>MAFNPAPKAVQENHHVDYVIRFNYGDIDTPEAIKKFEVLLLELSEVGLQTEVRQGDENSLFVFVRAASKKKLKRAVYQSRVRDWLYGVRNTEPEPASSAKPQSEAERLLVIYHLITVPKAEGGAGITPRHGEWKNVDAIFPLHDEETNRQCMREWSKKTFLSTEDLDRIRNTFGEHVGFYFAFLQSYFRFLMFPAAFGFSCWLLLGSFSIIYTVVNCLWCIVFIEYWKRQEEDLSCRWQTKGVSAVHEKRAEFKPEKEIRDESTGEVRGVFPATKRMYRQLLQVPFALLAAVALGAIIATCFAIEIFISEVYNGPLKGYLVFIPTILVSALIPTMSAVLLTVATKLNDYENYETQDAYKVALTQKIFVVNFITSYLPIILTAFVYVPFASRIVPYLDVFHLTVRPFVSKEHAIKARTEFSINPDRLRKQVIYFTVTAQIVGFALETIVPFVKQRVFREYKEYTKKQHAKAEPGNGAGEKKTVSLGDDEDEARFLTRVRNEAELEDYDVTDDLREMCIQFGYLALFSPVWPLVPVSFLINNWVELRSDFFKICVECKRPWPQRADTIGPWLDSLGFLSWVGSITSSALV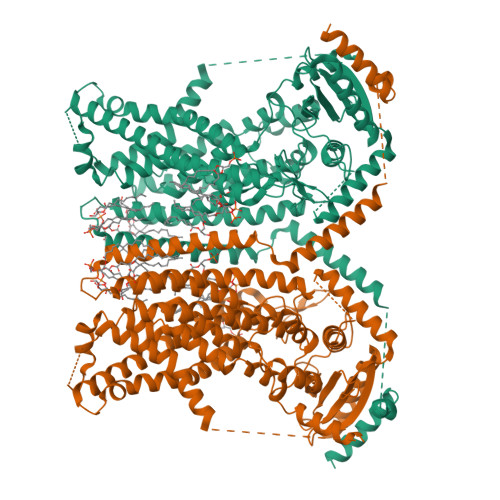YMFSNGHEGPNGEPTTIRCWALLLTIFFSEHLYLIVRYAVRSALAKLEPPNTRRERIERFMMRKRYLDTVLSAESDDDADEVKGVVSSIPPSEITRESLEQDARDWSKQGTDPTERFWMRQRGWKESAEVGLSLITKAKGDETKKQQ[2x]(1S)-N-(7-chloro-6-{4-[(3R,4R)-4-hydroxy-3-methyloxolan-3-yl]piperazin-1-yl}isoquinolin-3-yl)-6-oxaspiro[2.5]octane-1-carboxamide 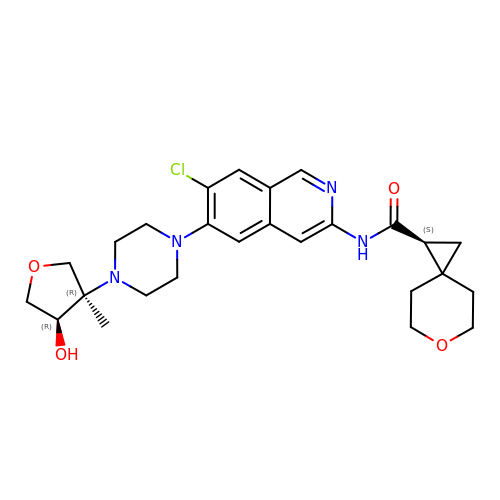| C26 H33 Cl N4 O4 | ISEBFQYGEPKLRU-RZTXVSJASA-N> EVCSEQAETGPCRAMISR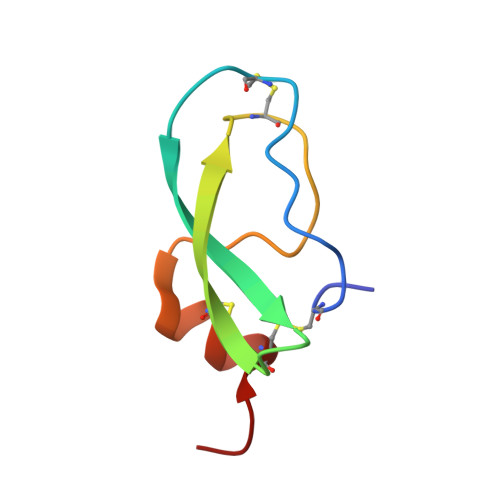WYFDVTEGKCAPFFYGGCGGNRNNFDTEEYCMAVCGSAI>KDDMKAAEQYQGAASAVDPAHVVRTNGAPDMSESEFNEAKQIYFQRCAGCHGVLRKGATGKPLTPDITQQRGQQYLEALITYGTPLGMPNWGSSGELSKEQITLMAKYIQHTPPQPPEWGMPEMRESWKVLVKPEDRPKKQLNDLDLPNLFSVTLRDAGQIALVDGDSKKIVKVIDTGYAVHISRMSASGRYLLVIGRDARIDMIDLWAKEPTKVAEIKIGIEARSVESSKFKGYEDRYTIAGAYWPPQFAIMDGETLEPKQIVSTRGMTVDTQTYHPEPRVAAIIASHEHPEFIVNVKETGKVLLVNYKDIDNLTVTSIGAAPFLHDGGWDSSHRYFMTAANNSNKVAVIDSKDRRLSALVDVGKTPHPGRGANFVHPKYGPVWSTSHLGD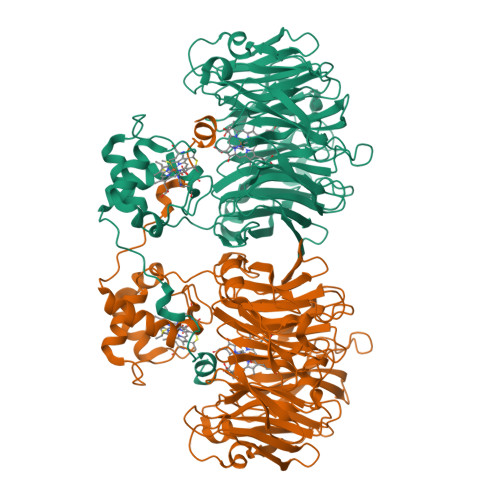GSISLIGTDPKNHPQYAWKKVAELQGQGGGSLFIKTHPKSSHLYVDTTFNPDARISQSVAVFDLKNLDAKYQVLPIAEWADLGEGAKRVVQPEYNKRGDEVWFSVWNGKNDSSALVVVDDKTLKLKAVVKDPRLITPTGKFNVYNTQHDVY[2x]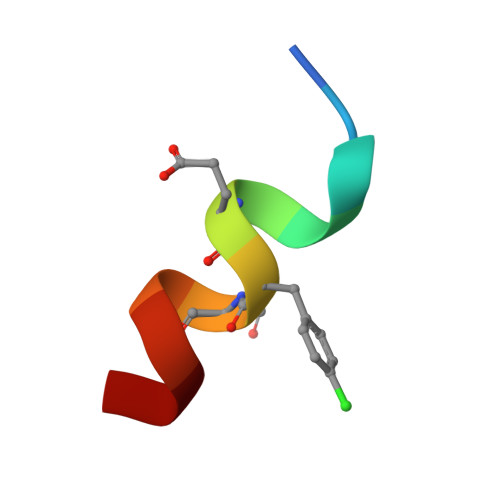> EFWYVEXEKLLR>[2x]GAMKVLARIFKETELRKLKVLGSGVFGTVHKGVWIPEGESIKIPVCIKV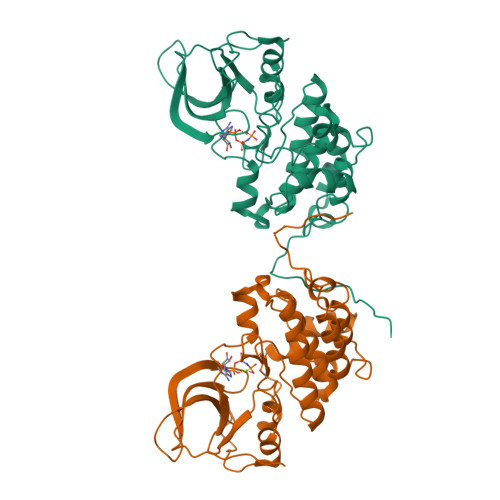IEDKSGRQSFQAVTDHMLAIGSLDHAHIVRLLGLCPGSSLQLVTQYLPLGSLLDHVRQHRGALGPQLLLNWGVQIAKGMYYLEEHGMVHRNLAARNVLLKSPSQVQVADFGVADLLPPDDKQLLYSEAKTPIKWMALESIHFGKYTHQSDVWSYGVTVWELMTFGAEPYAGLRLAEVPDLLEKGERLAQPQICTIDVYMVMVKCWMIDENIRPTFKELANEFTRMARDPPRYLVIKRESGPGIAPGPEPHGLTNKKLEEVELEPELDLDLDLEAEE>LLVVGPKFIRANQEYTLVISNFNSQLSKVDLLLKLEGETDNGLSVLNVTKMVDVRRNMNRMINFNMPEELTAGNYKITIDGQRGFSFHKEAELVYLSKSISGLIQVDKPVFKPGDTVNFRVILLDTELKPPARVKSVYVTIRDPQRNVIRKWSTAKLYAGVFESDLQIVPTPMLGVWNISVEVEGEELVSKTFEVKEYVLSTFDVQVMPSVIPLEEHQAVNLTIEANYHFGKPVQGVAKVELYLDDDKLNQKKELTVYG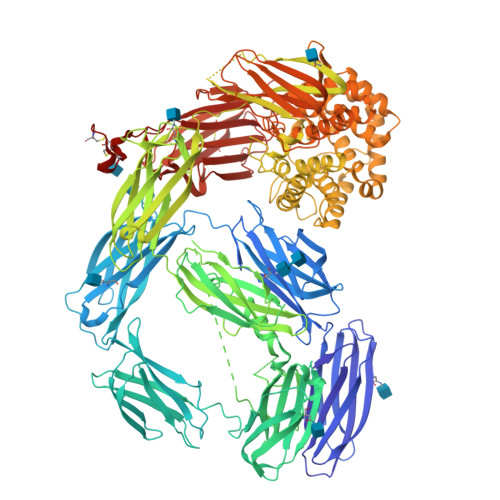KGQVELRFDNFAMDADQQDVRVKVSFIEQYTNRTVVKQSQITVYRYAYRVELIKESPQFRPGLPFKCALQFTHHDGTPAKGITGKVEVSDVGFETTTTSDNDGLIKLELQPSEGTEQLGINFNAVDGFFFYEDVNKVETVTDAYIKLELKSPIKRNKLMRFMVTCTERMTFFVYYVMSKGNIIDAGFMRPNKQTKYLLQLNATEKMIPKAKILIATVAGRTVVYDYADLDFQELRNNFDLSIDEQEIKPGRQIELSMSGRPGAYVGLAAYDKALLLFNKNHDLFWEDIGQVFDGFHAINENEFDIFHSLGLFARTLDDILFDSANEKTGRNALQSGKPIGKLVSYRTNFQESWLWKNVSIGRSGSRKLIEVVPDTTTSWYLTGFSIDPVYGLGIIKKPIQFTTVQPFYIVENLPYSIKRGEAVVLQFTLFNNLGAEYIADVTLYNVANQTEFVGRPDTDLSYTKSVSVPPKVGVPISFLIKARKLGEMAVRVKASIMLGHETDALEKVIRVMPESLAQPKMDTSFFCFDDYKNQTFPFNLDINKKADNGSKKIEFRLNPNLLTMVIKNLDNLLAVPTGCGEQNMVKFVPNILVLDYLYATGSKEQHLIDKATNLLRQGYQNQMRYRQTDGSFGVWEKSGSSVFLTAFVATSMQTASKYMNDIDAAMVEKALDWLASKQHSSGRFDETGKVWHKDMQGGLRNGVALTSYVLTALLENDIAKVKHAVVIQNGMNYLSNQLAFINNPYDLSIATYAMMLNGHTMKKEALDKLIDMSISDNNKKERYWGTTNQIETTAYALLSFVMAEKYLDGIPVMNWLVNQRYVTGSFPRTQDTFVGLKALTKLAEKISPSRNDYTVQLKYKKNTKYFNINSEQIDVQNFLEIPEDTKKLEINVGGIGFGLLEVIYQFDLNLVNFEHRFKLDLEKQNTGSDYELRLRVCANYIPELTDSQSNMALIEVTLPSGYVVDRNPISEQTTVNPIQNMEIRYGGTSVVLYYYKMGTERNCFTVTAYRRFKVALKRPAYVVVYDYYNTNLNAIKVYEVDKQNVCEICEEEDCPAECHHHHHH[3x]> EIETIVRESEANRIQAQTWFSHPEKSKVSFRYDERETSSIRSISIETFLSFYSSKFNREPYSVLDIGCGQG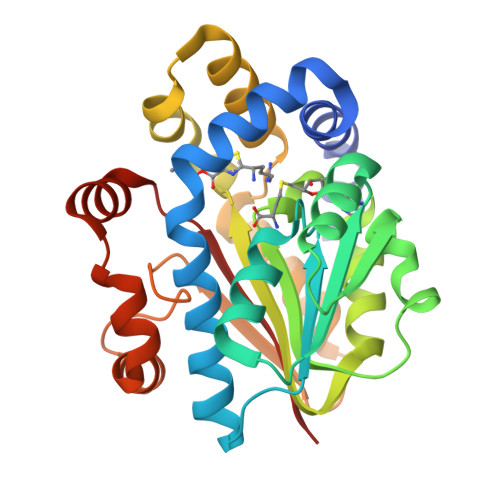QVIQYLNSRFQKIELTGIDSSAQAISSAKKLGINASFICSNAENIMQYVSKKQDIIFIHLCFGLFKNPIAIVNTLIHLLSDQSCIYIVDLDRNSLGEGLNTAQSREEEAYLKDQYRASLTMEEFKQLLHVVTKEQHGVSFHVGNSFIGGFDETSSQFFSLMRNRNLQDALRTSVGEQLKQSQMPALLHGWIIKNK>MHHHHHHMIEELGKIDRIIQESVPGKQITLAHVIAAPIEAVYEALGVDHEGAIGVVSLTPNETAIIAADIAGAAANIDICFVDRFTGSVMFSGDIQSVETSLEDILEYFKNSLGFSTVPL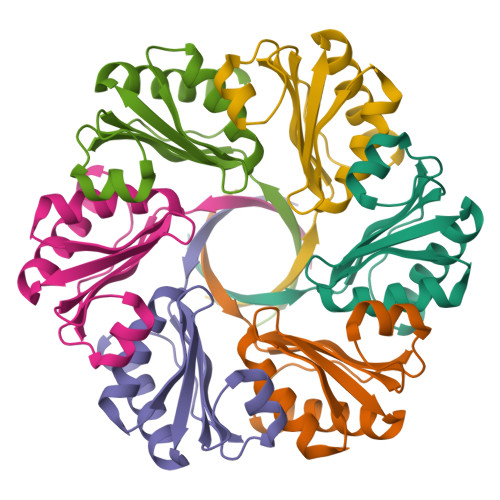TKS[6x]>MEKEDSGFFSTSFKYVLSACIASFIFGYQVSVLNTIKNFIVVEFEWCKGEKDRLNCSNNTIQSSFLLASVFIGAVLGCGFSGYLVQFGRRLSLLIIYNFFFLVSILTSITHHFHTILFARLLSGFGIGLVTVSVPMYISEMTHKDKKGAYGVMHQLFITFGIFVAVMLGLAMGEGPKADSTEPLTSFAKLWWRLMFLFPSVISLIGILALVVFFKEETPYFLFEKGRIEESKNILKKIYETDNVDEPLNAIKEAVEQNESAKKNSLSLLSALKIPSYRYVIILGCLLSGLQQFTGINVLVSNSNELYKEFLDSHLITILSVVMTAVNFLMTFPAIYIVEKLGRKTLLLWGCVGVLVAYL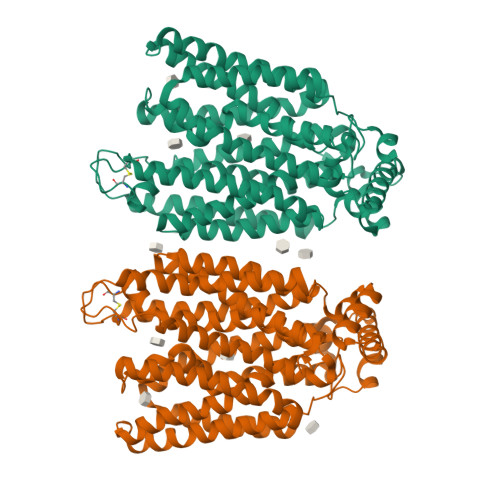PTAIANEINRNSNFVKILSIVATFVMIISFAVSYGPVLWIYLHEMFPSEIKDSAASLASLVNWVCAIIVVFPSDIIIKKSPSILFIVFSVMSILTFFFIFFFIKETKGGEIGTSPYITMEERQKHMTKSVVENLYFQ[4x]> MNQIEPGVQYNYVYDEDEYMIQEEEWDRDLLLDPAWEKQQRKTFTAWCNSHLRKAGTQIENIEEDFRNGLKLMLLLEVISGERLPKPDRGKMRFHKIANVNKALDYIASKGVKLVSIGAEEIVDGNVKMTLGMIWTIILRFAIQDISVEETSAKEGLLLWCQRKTAPYRNVNIQNFHTSWKDGLGLCALIHRHRPDLIDYSKLNKDDPIGNINLAMEIAEKHLDIPKMLDAEDIVNTPKPDERAIMTYVSCFYHAFAGAEQAETAANRICKVLAVNQENERLMEEYERLASELLEWIRRTIPWLENRTPEKTMQAMQKKLEDFRDYRRKHKPPKVQEKCQLEINFNTLQTKLRISNRPAFMPSEGKMVSDIAGAWQRLEQAEKGYEEWLLNEIRRLERLEHLAEKFRQKASTHETWAYGKEQILLQKDYESASLTEVRALLRKHEAFESDLAAHQDRVEQIAAIAQELNELDYHDAVNVNDRCQKICDQWDRLGTLTQKRREALERMSERVRNFEDPAANKARKEAELAAATAEQ;> GSSKLLETIDQLHLEFAKRAAPFNNWMEGAMEDLQDMFIVHSIEEIQSLITAHEQFKATLPEADGERQSIMAIQNEVEKVIQSYNIRISSSNPYSTVTMDELRTKWDKVKQLVPIRDQSLQEELARQHANERLRRQFAAQANAIGPWIQNKMEEIARSSIQITGALEDQMNQLKQYEHNIINYKNNIDKLEGDHQLIQEALVFDNKHTNYTMEHIRVGWELLLTTIARTINEVETQILTRDAKGITQEQMNEFRASFNHFDRRKNGLMDHEDFRACLISMGYDLGEAEFARIMTLVDPNGQGTVTFQSFIDFMTRETADTDTAEQVIASFRILASDKPYILAEELRRELPPDQAQYCIKRMPAYSGPGSVPGALDYAAFSSALYGESDL;> GPTVGGQLGTAGQGFSYSKSNGRGGSQAGGSGSAGQYGSDQQHHLGSGSGAGGTGGPAGQAGRGGAAGTAGVGETGSGDQAGGEGKHITVFKTYISPWERAM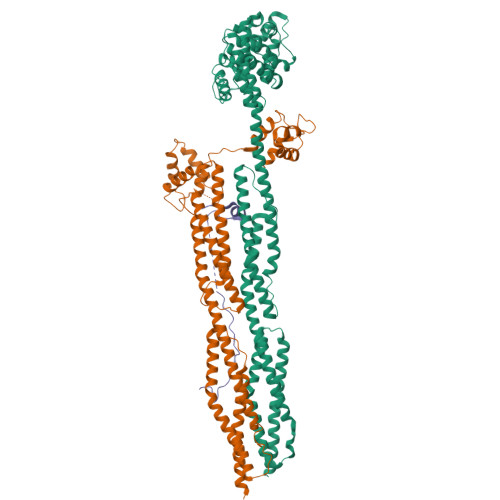GVDPQQKMELGIDLLAYGAKAELPKYKSFNRTAMPYGGYEKASKRMTFQMPKFDLGPLLSEPLVLYNQNLSNRPSFNRTPIPWLSSGEPVDYNVDIGIPLDGETEEL>[2x]MKAPSYHVVRGDIATATEGVIINAANSKGQPGGGVCGALYKKFPESFDLQPIEVGKARLVKGAAKHIIHAVGPNFNKVSEVEGDKQLAEAYESIAKIVNDNNYKSVAIPLLSTGIFSG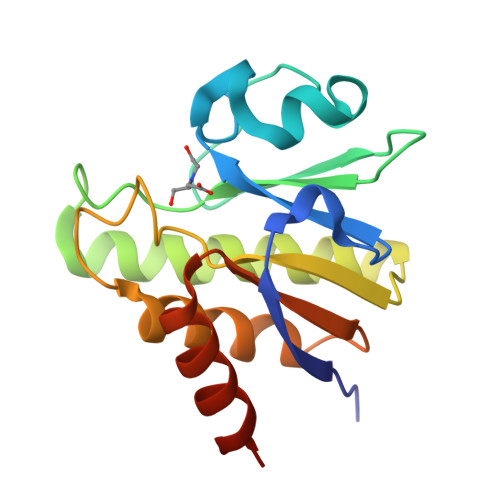NKDRLTQSLNHLLTALDTTDADVAIYCRDKKWEMTLKEAVARREHHHHHH>[4x]GAMSPNSTLYSTGRPAGRFTLRPMRHEDAAMVHRWVTQEYARFWGMQDNSIEQVAAFYHQLTAHNPHAALIGCCNDQPVFLMEFYKASEDDIGKFYAAQPGDYGMHLLIAPATHPVQQFSWQVFSTVIDFM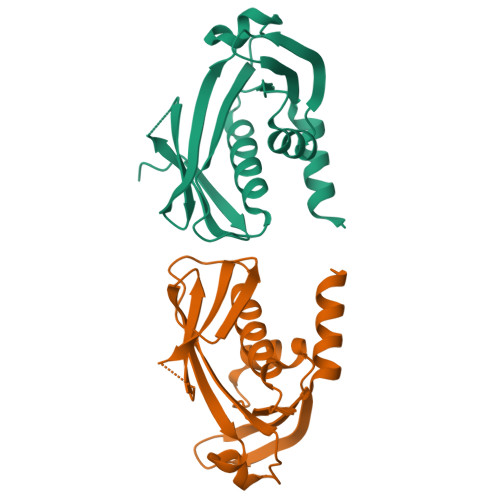FSLPEVKRVVVEPDERNTKIHRLNKRAGFCYQHTIDMGHKTAWLAFCQRENYQQALLKESLNMNDTHLLQAGTWLTGDNWAEANRLLIRKAIAEFAHEKIVTPAECAHGRYSLAVPGSETEYQFTASRLALDHWEIDAASLTKQENGHPLALDALQFITEFNEVIGIPQALLATYMEEISSTLCSSVFKLQKNNPDSRALVNADFQTVESSMTEGHPCFVANNGRIGFDARDYLAYAPEAATPVNLIWVAVHRRNAHFSSLSDLQYERLMREELGQSTVEQFNAQLTEKGLTHADYLFMPVHPWQWQNKLLTVFAADIANNDIVWLGVGDDQYQAQQSIRTFFNRSHPNKRYVKTALSVLNMGFMRGLSPYYMATTPAINEWLQDLVAGDEWLQRCDFRILREVAAVGYHNRHYEKAIKGDSAYKKMFAALWRDNPVAELKPGQRLMTMASFLHVDHHQKALLPALIADSGLAAERWVERYLSCYLSPLLHCFYQHDLVFMPHGENLILLLENNVPVSAYMKDIGEEIAVMNPDAVLPEKVQRLAVDVPENLKLLSVFTDVFDCIFRFISAILHQSATLPEEQFWQAVARCVKEYQQAHPHLASKFSRYDMFAPEFTRSCLNRLQLANNQQMINLSDPAENLKFAGTLVNPIARWR>[2x]MTTQAPTFTQPLQSVVVLEGSTATFEAHISGFPVPEVSWFRDGQVISTSTLPGVQISFSDGRAKLTIPAVTKANSGRYSLKATNGSGQATSTAELLVKAETAPPNFVQRLQSMTVRQGSQVRLQVRVTGIPTPVVKFYRDGAEIQSSLDFQISQEGDLYSLLIAEAYPEDSGTYSVNATNSVGRATSTAELLVQGETREEF;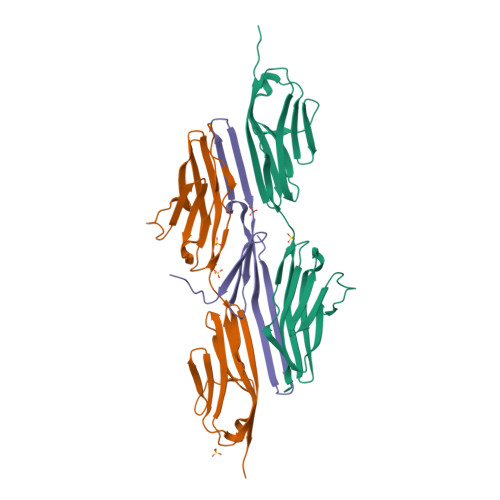> MATSELSSEVSEENSERREAFWAEWKDLTLSTRPEEGSSLHEEDTQRHETYHQQGQSQVLVQRSPWLMMRMGILGRGLQEYQLPYQRVLP> MGSKCSNSGIECDSSGTCINPSNWCDGVSHCPGGEDENRCVRLYGPNFILQVYSSQRKSWHPVCQDDWNENYGRAACRDMGYKNNFYSSQGIVDDSGSTSFMKLNTSAGNVDIYKKLYHSDACSSKAVVSLRCIACGVNLNSSRQSRIVGGESALPGAWPWQVSLHVQNVHVCGGSIITPEWIVTAAHCVEKP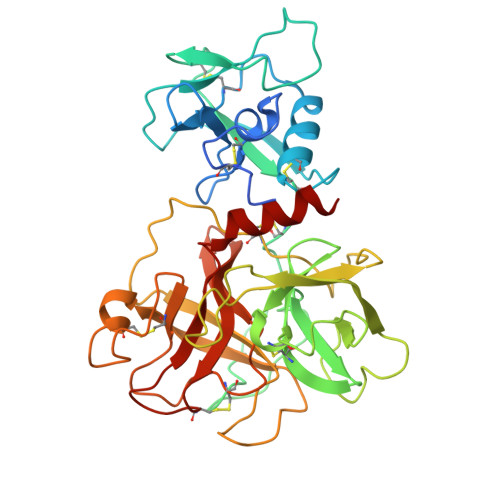LNNPWHWTAFAGILRQSFMFYGAGYQVEKVISHPNYDSKTKNNDIALMKLQKPLTFNDLVKPVCLPNPGMMLQPEQLCWISGWGATEEKGKTSEVLNAAKVLLIETQRCNSRYVYDNLITPAMICAGFLQGNVDSCQGDAGGPLVTSKNNIWWLIGDTSWGSGCAKAYRPGVYGNVMVFTDWIYRQMRADG The mycobacterial HTH-transcriptional regulator (EthR) has been reported to be a facilitator for the resistance of the second-line tuberculosis drug, ethionamide. Studies of the resistance mechanism of ethionamide revealed that an increase in the expression of HTH-Transcriptional regulator, EthR, reduces transcription and the level of active EthA protein, and results in resistance by M. tuberculosis. The discovery of this transcriptional regulator led to the notion of controlling EthA expression levels by targeting EthR and thus boosting the bactericidal effect of ethionamide. EthR binding site is characterized by a long hydrophobic tunnel surrounded mostly by hydrophobic residues, many of which are aromatic, plus four polar amino acids and a basic residue.

We then managed to obtain X-ray crystal structures for compounds 1, 2, 3, 5, 6, 7, 10, and 12 bound to EthR. The EthR-compound 1 co-crystal structure confirms the occupancy of the compound in the EthR binding site. Compound 1 is active against both EthR (IC50 ≈12 μM) and InhA (62% inhibition at 100 μM), confirming the computational predictions. Interestingly, this compound was identified solely from structure-based predictions. Even though an attempt to obtain a co-crystal structure of the compound with InhA was unsuccessful, the docking LEI values for the compound to both enzymes (EthR: 1.58 and InhA: 1.11) indicate high binding affinity. Another common feature shared between several of the compounds (1, 2, 3, 7, and 10) is the presence of a ketone that forms a hydrogen bond with N176 in all but compound 3. Thiophenes and thioethers are present in compounds 1, 8, and 10 and are known to be substrates for EthA.

> MDIEFTTSAASQASLPRGRRTARPSGDDRELAILATAENLLEDRPLADISVDDLAKGAGISRPTFYFYFPSKEAVLLTLLDRVVNQADMALQTLAENPADTDRENMWRTGINVFFETFGSHKAVTRAGQAARATSVEVAELWSTFMQKWIAYTAAVIDAERDRGAAPRTLPAHELATALNLMNERTLFASFAGEQPSVPEARVLDTLVHIWVTSIYGENRGSHHHHHH>[2x]WIMSQTNANDLRNNEVFFISPSNNTNKVLDKISQSEVKLWNKLSGANQKWRLIYDTNKQAYKIKVMDNTSLILTWNAPLSSVSVKTDTNGDNQYWYLLQNYISRN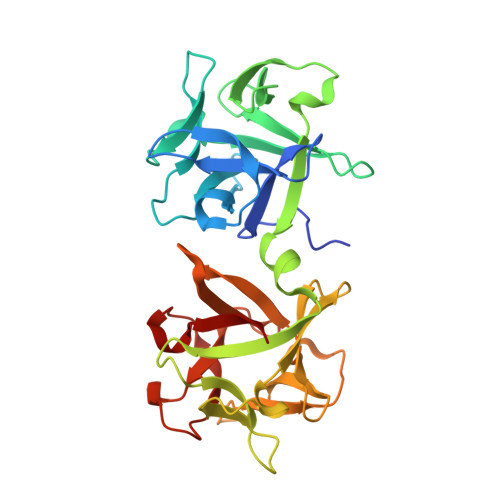VIIRNYMNPNLVLQYNIDDTLMVSTQTSSSNQFFKFSNCIYEALNNRNCKLQTQLNSDRFLSKNLNSQIIVLWQWFDSSRQKWIIEYNETKSAYTLKCQENNRYLTWIQNSNNYVETYQSTDSLIQYWNINYLDNDASKYILYNLQDTNRVLDVYNSQIANGTHVIVDSYHGNTNQQWIINLI>MYKDLEGKVVVITGSSTGLGKSMAIRFATEKAKVVVNYRSKEDEANSVLEEIKKVGGEAIAVKGDVTVESDVINLVQ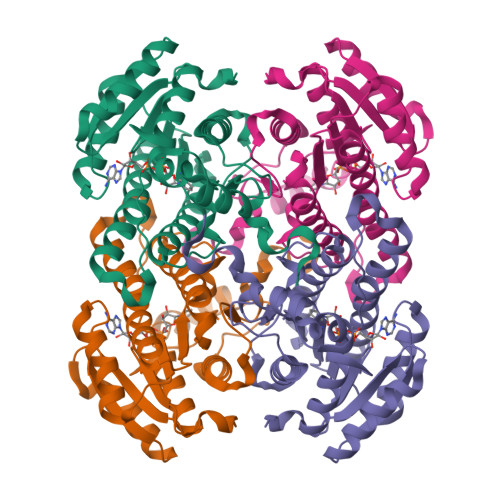SAIKEFGKLDVMINNAGLENPVSSHEMSLSDWNKVIDTNLTGAFLGSREAIKYFVENDIKGTVINMSSVHEKIPWPLFVHYAASKGGMKLMTKTLALEYAPKGIRVNNIGPGAINTPINAEKFADPEQRADVESMIPMGYIGEPEEIAAVAAWLASSEASYVTGITLFADGGMTLYPSFQAGRG[4x]> MYAHVVSWTLFLHVFFFFLSLSRTLFFFFFFFVCLFFPFLCVYLEEEMLRRLVSSHGCSNGGGTNGGRCVRPVKEEPPVFSSLVLQRRFSFKYATKLQHDEMRQPFYIHEKRHGIFSNEKNIRKSRRGLPFITPLYTRHMNLWETDTDASKNRFFRGYVFGQRELHQLLGRPHGFEANNTDGSNDISAYEMTTDQRYKGIPRPAITNLHYEPEWNYTLYRAGTHGSQLSNPRSPLTAEVLGDELMKIRDIKSFDHCKAWFDRLQYLIKLHYDAVGDIGEFKSRHTQHVHEFFVAFHDALSSFDFGDSYLFEQFHAARPSELTDLFGIFLEMEANYVHEDYCPRCSLPYSTTRYCGEGDANTPFRKHRGRWAPHQRWGREWYAVVARRAEALWYRATEDPYFGTPQHTQRQAEALLRVYVQTKQRGKAIDFMNALRGSKEFLLGSICITPEMQESYDRLLDTTPHPHLLTNGFTLESNAAKYTGEVQKVPFSPLQFRIDMEMNKYRRQQKEEGAVRVPPAMWRIDTSAIVPYKVDPKTKRVINWREVKEGIEKSFLSTGLPKEAYTGSEWREMLHLKSIIAGRAAKAAELERRLHTDKVKLLEVSSKSKIASETNTSTGSSNSSSIIFPDKDGYHVFDTSVASLRPFGVSQSGAVFQSVTHTYPSPHAVLYNDPVHGKQFILDTTNESCHLFGGFEHGDRLLIRARKIDKNDNNPNSVLAVKGNEFEVIVVGVNKEGSDSEWQLCAMHVDPALQREYGLVFLGTDCVDIHERWASVRYAAAAPHVKGRVTLLEERRTAREESLGQIVGVRDGVLFVQWRLLRGGGSEMDRSVAEPIGTVEQVRNAYQITEQGVEELMHPPSWRTPFRNDFAEERLEELRQAPFKRENWVSLIQGRYTPKLKRFGYTQHTTMDDFETKEYKDRLLSKQFFHNPQAFEVIPDRRDRAVTFGGKWEYQRTHGLPTVDRNELENGWSEVEAVTDAEMHVIEQALRDISGRRPGNFIKSPTKKNTLQLNESWWEPLEFGWEQHNKEQKA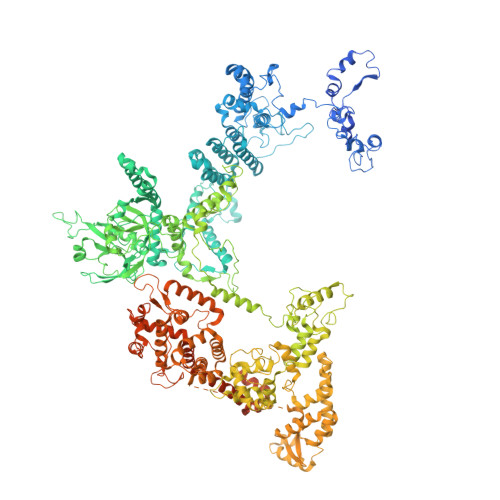LVDPTEQRLIDSASLPFGGKIPPFGTTIGIGERIREIAEDYAKGFGLGPHGHSPSHDTCQYNTLNAEEDRVRELGYKDALVRLFDEKMADKDVHQWAVEQCADGEADVRQLLLSLHEWRERGRPPSLMLLQVLSKYLEQEIAAFNEGVPSSVPKLSLQTVDGTLSPSGNSGERSGTIWADVEPTAYALQYASQANHSSLDEPFILQLLKSAQLGGRNAQFTDPFYNAYLENSVVSEFQLGLAALAGKGVSPSLLAQKISQLHRGSVRLSGNVIPFVKSRELAHLLERMGLSSENIAVVTRGLANCPEQESVGDDFAVPVSVILSWGGPGSGSSTNAADRKGNATQSRNELQRKGSAALSSAIRQLGQKRSSSKNWQNEDKMMVHVIEELALRDDGLVMDIQYIVRENRRNPVLRHEFFAALLPVFAGKHEKVAQLYDEYCEGKYVPNITLAIEAFIAFLCNVTKHADVYPGSSYFDVDTTNGPNAGQYISLKLLDPLDGPFIFDNIKAEHIETVERFKQHGIQVGPVRAPATGFIAANSKSLSYFTRRPEEVVYVSTDADQGLRRSLERSAHYKTIAASPAMQFLLHTQNGAGLVATFNRFFYRTMPMLSFYQRILKHYSDNVQPLRQKAQNSVRGLARVLENERSAAMEEFRRNSERYWRNVLEGRSVEQAMGGSGGSGGGGGGTTPPVSSSPSQSSQEAMAADVARAIGSGRTGDQKGGAARQQQQQQQRTAGDDGGVRTTFASRKGGSRSMTDLLSKLNKPKGSNTSGTAKGPTKRGNPKSHTDGGRGAKP>[2x]MVLDLDLFRVDKGGDPALIRETQEKRFKDPGLVDQLVKADSEWRRCRFRADNLNKLKNLCSKTIGEKMKKKEPVGDDESVPENVLSFDDLTADALANLKVSQIKKVRLLIDEAILKCDAERIKLEAERFENLREIGNLLHPSVPISNDEDVDNKVERIWGDCTVRKKYSHVDLVVMVDGFEGEKGAVVAGSRGYFLKGVLVFLEQALIQYALRTLGSRGYIPIYTPFFMRKEVMQEVAQLSQFDEELYKVIGKGSEKSDDNSYDEKYLIATSEQPIAALHRDEWLRPEDLPIKYAGLSTCFRQEVGSHGRDTRGIFRVHQFEKIEQFVYSSPHDNKSWEMFEEMITTAEEFYQSLGIPYHIVNIVSGSLNHAASKKLDLEAWFPGSGAFRELVSCSNCTDYQARRLRIRYGQTKKMMDKVEFVHMLNATMCATTRTICAILE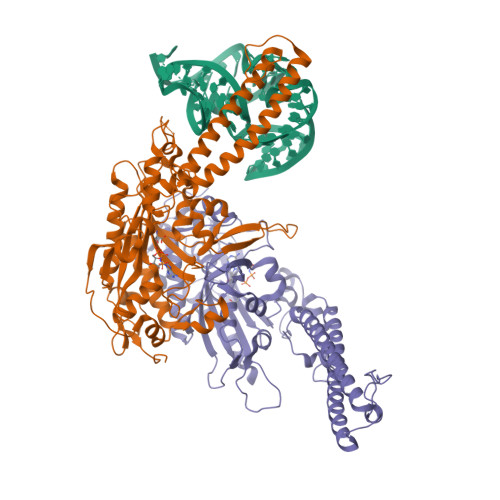NYQTKKGITVPEKLKEFMPPGLQELIPFVKPAPIEQEPSKKQKKQHEGSKKKAAARDVTLENRLQNMEVTDALEHHHHHH>REVLTGGHSVSAPQENRIYVMDSVFMHLTESRVHVYDYTNGKFLGMVPTAFNGHVQVSNDGKKIYTMTTYHERITRGKRSDVVEVWDADKLTFEKEISLPPKRVQGLNYDGLFRQTTDGKFIVLQNASPATSIGIVDVAKGDYVEDVTAAAGCWSVIPQPNRPRSFMTICGDGGLLTINLGEDGKVASQSRSKQMFSVKDDPIFIAPALDKDKAHFVSYYGNVYSADFSGDEVKVDGPWSLLNDEDKAKNWVPGGYNLVGLHRASGRMYVFMHPDGKEGTHKFPAAEIWVMDTKTKQRVARIPGRDALSMTIDQQRNLMLTLDGGNVNVYDISQPEPKLLRTIEGAAEASLQVQ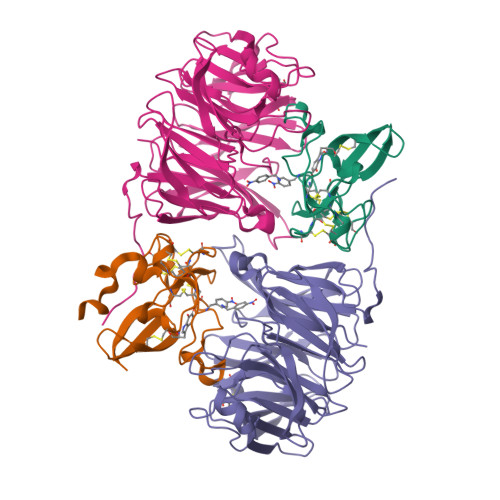FHPVGGT[2x];>AGGGGSSSGADHISLNPDLANEDEVNSCDYWRHCAVDGFLCSCCGGTTTTCPPGSTPSPISWIGTCHNPHDGKDYLISYHDCCGKTACGRCQCNTQTRERPGYEFFLHNDVNWCMANENSTFHCTTSVLVGLAKN[2x]(2S)-2-[(3-{3-[(2,4-diamino-6-ethylpyrimidin-5-yl)oxy]propoxy}phenyl)methyl]-3,3-difluoropropanoic 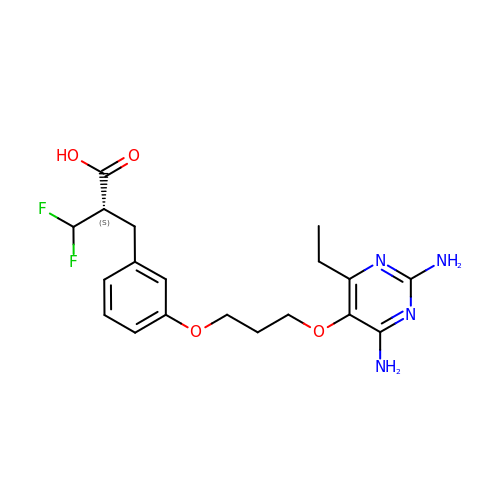acid | C19 H24 F2 N4 O4 | QMHPAIITCHQDEY-CYBMUJFWSA-N> MFRRLSSSARAVVAARFYTPPEGLKKLYASDFENSKYPLNIVPSDSVLFAKFLYKAAEEKGNFDNILSDFQKIAAAASKLPIFWERTAVVEKIPEFKQLSEPTFFTLVWMQNNGMLELIQEVAEVYETFVNAKQKKAVAKIF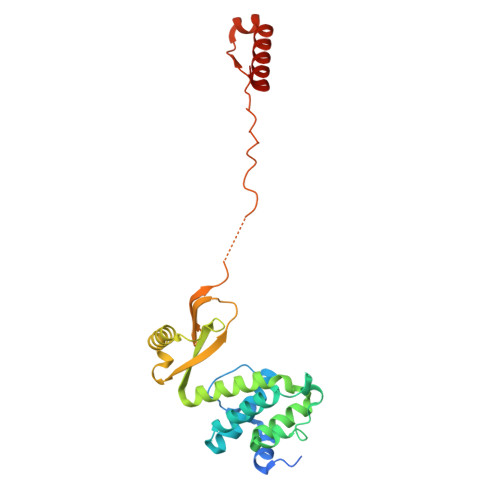VAPGGEKNVEEARRVAEELHKGLKELADYTLVLKTVVDRTIVKGFAVELAGQYVNKAEGQQKQAGRADEVDYTNLPAPKPQKTVWDDNIETEVLRKYLDGLSQYDMEEAKYGV> MGSSHHHHHHSQDMEAAIEFDEIVKKLLNIYINDICTTGEKRLLNNYEKSILDRIYKSCEYIKKNYELDFNSMYNQININDITTSDIKSKIIEALLIDSRP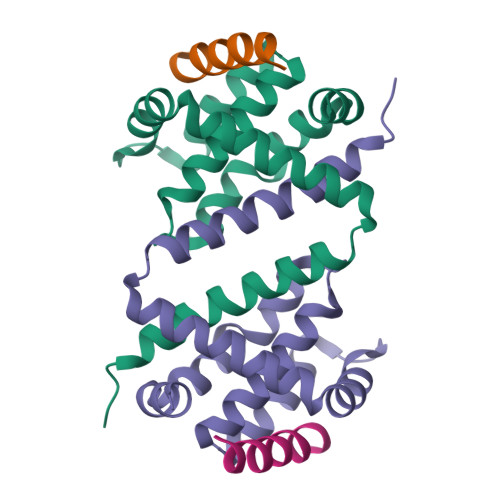SVKLATLSFISLIAEKWGEKNRAKIMEILSNEIVEKISNNGKDFIDFIDRDDDDIVDDYVLITNYLK;> DMRPEIWIAQELRRIGDEFNAYYARR> MLQKRIPQIICTLLLLGSFSQIKAQDRVPFDQGKKYTLAKVSVVGKISFNEQTVVTFSGLQKGQEITVPGEEITSAIKKLGKLGLFDEIAFYINKVENDSIYLDLNIVELPKLNEVKITGVKKSKVEGLIKDNNLTKNKIVNENLITTTKNYIENKYKKDGFYNTKVVITTTPDTTAGNQVNMLVRVDKGDKVKISSIDFTGNKQLSDSKLRAAMKDTKQKNVLRVFKASKFIPEKYKTDLEKVIASYKEKGYRDARIIYDSVIYNKKKNMLAIKIDVEEGNKYYFGNIKFLGNTVYSDQQLNRYLGIKKGETYNGVLLEKRIADNTKPDGEDITNLYQNNGYLFSKINAVEVKTVNDTIDFEIRITEGPIAYFNKIYVTGNDKTNDHVIYRELRTKPGNKYSKEELVRTIREIGQLGFFDPESIKPEFRNVDPAAGTVDIEYQLVEKGSSQVELQGGYGGGGFIGTLGLSFNNFSARKLFDKDAYKPLPMGDGQKVALRLQGSTYFQTYSLSFSEPWFGGKKPVQFSSSISYSKQFNYNYSSRDVNRNQSFNIFTVQVGLAKRLTVPDDYFVLSQSVSYQHYDLNNYYTGLFTFGNGASRNLAYTIGLSRSNKGVNPIFPTYGSEFSISAKVTPPYSLFNNINYGDLQNQKEYKTQYTGTTTTTGIDGQAINPGDYTKTETVNGQSGTVSVGSDYKSADTDVGKVDQKKYNWLEYYKVKFKADWYTKIYGKLVLRTLTEFGFLGAYDQSRGVVPFERFYLGGDGMANYSMDGRETIQLRGYPNNSLTPIIEDRNSSRYGQQIGATIYNKFSMELRYPITLKSSASIYALTFLEAGSSYPTFKDYNPFDLNRSAGAGLRVFMPAFGLLGIDFGYGFDALPGSTTNKANGWETHFIIGQQF;> MKNKLGVFVVCLFCQIMLGQNGTRKSLHGQVTNKSLAIESGYVMNINAKS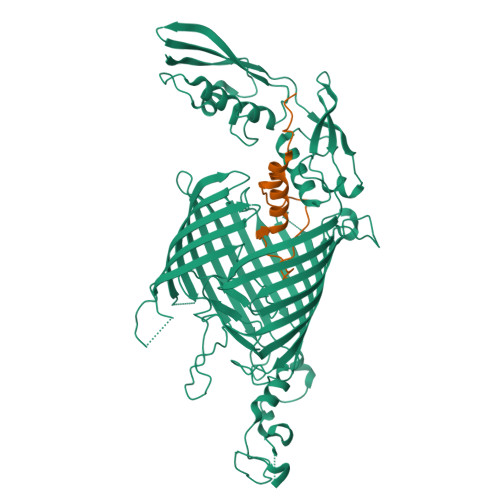RTFIGPGGLFDILAQPKDTLLFTGIAFQSKKIVLTEKDCSQILFSVSLDLVSNELKEVLVRKDLKVKSLDSNTQKYVDMQFEDDRQSTAKNTVMYSDQTIKYGTDFVRIFKDVKKLLSKNNEKEEVISDIAFVEYSKANFKPDFYTKTLGLKPDEVDLFLMFCSNDPESKRHLNEDQKFELIDFLINKNAEFKKVNAAQ Calcium-independent phospholipase A2β (iPLA2β, also known as PLA2G6A or PNPLA9) hydrolyses membrane phospholipids to produce potent lipid second messengers. The sequence can be divided into three parts: the N-terminal domain, the ankyrin repeat (AR) domain (ANK) and the catalytic domain (CAT). The lipid hydrolysis is executed by a Ser-Asp catalytic dyad in close spatial proximity to a glycine-rich motif. Here, we present the crystal structure of a mammalian iPLA2β, which revises previous structural models and reveals several unexpected features critical for regulation of its catalytic activity and localization in cells.

The structure of the short variant of iPLA2β (SH-iPLA2β, 752 amino acids) was solved by a combination of selenomethionine single-wavelength anomalous diffraction (SAD) with molecular replacement (MR) using two different protein models. The sequence assignment was guided by position of 51 selenium peaks and the structure was refined using 3.95 Å resolution data. The electron density map reveals nine ARs in the structure of SH-iPLA2β, instead of the previously predicted eight. The crystallographic asymmetric unit is formed by a dimer of iPLA2β. In contrast with the original hypothesis of ANK-mediated oligomerization, this dimer is formed through CAT domains. CAT domains interact through an extended, largely hydrophobic dimerization interface with a contact area of ~2,800 Å2 formed by three α-helices, several loops, including the long loop 554–570, and a part of the central β-sheet. Importantly, the active sites are in the immediate vicinity of the dimerization interface and in close spatial proximity to each other. By contrast, in iPLA2β, the active site cavity is wide open and can accommodate phospholipids with long polyunasturated fatty acid chains. In the crystal structure, it wraps around the CAT domain towards the predicted membrane-interacting surface. A single anomalous peak was consistently found near Trp293 of AR6.

>[2x]MQFFGRLVNTLSSVTNLFSNPFRVKEISVADYTSHERVREEGQLILFQNASNRTWDCILVSPRNPHSGFRLFQLESEADALVNFQQFSSQLPPFYESSVQVLHVEVLQHLSDLIRSHPSWTVTHLAVELGIRECFHHSRIISCANSTENEEGCTPLHLACRKGDSEILVELVQYCHAQMDVTDNKGETAFHYAVQGDNSQVLQLLGKNASAGLNQVNKQGLTPLHLACQMGKQEMVRVLLLCNARCNVMGPSGFPIHTAMKFSQKGCAEMIISMDSSQIHSKDPRYGASPLHWAKNAEMARMLLKRGCDVDSTSAAGNTALHVAVMRNRFDCVMVLLTYGANAGTPGEHGNTPLHLAISKDNMEMIKALIVFGAEVDTPNDFGETPAFMASKISKQLQDLMPISRARKPAFILSSMRDEKRIHDHLLCLDGGGVKGLVIIQLLIAIEKASGVATKDLFDWVAGTSTGGILALAILHSKSMAYMRGVYFRMKDEVFRGSRPYESGPLEEFLKREFGEHTKMTDVKKPKVMLTGTLSDRQPAELHLFRNYDAPEVIREPRFNQNINLKPPTQPADQLVWRAARSSGAAPTYFRPNGRFLDGGLLANNPTLDAMTEIHEYNQDMIRKGQGNKVKKLSIVVSLGTGRSPQVPVTCVDVFRPSNPWELAKTVFGAKELGKMVVDCCTDPDGRAVDRARAWSEMVGIQYFRLNPQLGSDIMLDEVNDAVLVNALWETEVYIYEHREEFQKLVQMLLSP>[2x]MLVLGLNGNFSAADTDVVPQLGEVFFHDSAASLIRDGELVAAVEEERLNRIKKTTKFPLNAVRECLALAGARPEDVDAVGYYFPENHIDTVLNHLYTEYPRAPLRYSRELIRQRLKEGLGWDLPDEKLVYVPHHEAHAYSSYLHSGMDSALVLVLDGRGELHSGTVYRAEGTRLEKLADYPVPKSLGGLYLNATYLLGYGFGDEYKVMGLAPWGNPETYRDTFAKLYTLQDNGEYELHGNIMVPNLVSPLFYAEGFRPRRKGEPFTQAHRDFAAALQETVEKIVLHILEYWAKTSGHSRLCFGGGVAHNSSLNGLILKSGLFDEVFVHPASHDAGAGEGAAYAAAASLGTLERPGKRLLSASLGPALGGREQIRARLADWAPLIDVEFPDDAVETAAGLL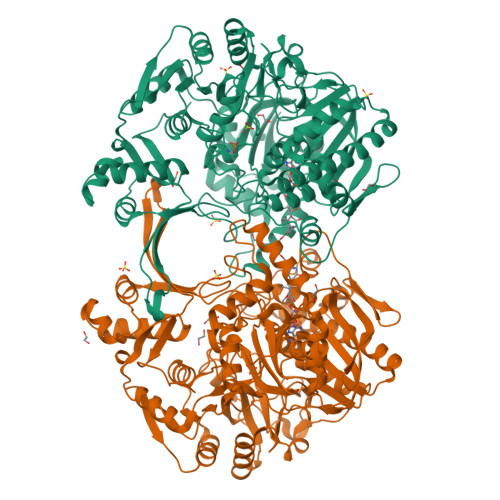AEGQVLGWAYGRSEFGPRALGHRSIVADARPEENRTRINAMVKKREGFRPFAPVVTAEAARDYFDLSGADGNHEFMSFVVPVLPERRTELGAVTHVDGTARVQVVSAESGERFHRLVRRFGELTGTPVLLNTSFNNNAEPIVQSLDDVVTSFLTTDLDVLVVEDCLVRGKASPDLGVLVPRFRPVTRLVERRTAGPDASAGAKTHEIHLDYDGGPSAKVSPELYELLGAVDGTTTLGDLAKTVGGLSDALATEVFALWEQRFLTLAPAGDIGPLADDGTRGH>[4x]MSDKTKTNEGFSRRSFIGSAAVVTAGVAGLGAIDAASATQKTNRASTVKGGFDYD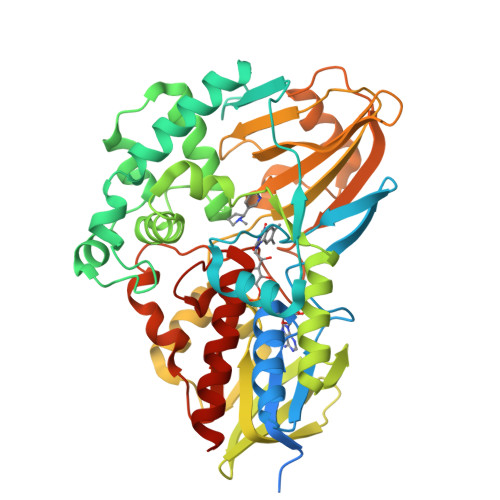VVVVGGGFAGATAARECGLQGYRTLLLEARSRLGGRTFTSRFAGQEIEFGGAWVHWLQPHVWAEMQRYGLGVVEDPLTNLDKTLIMYNDGSVESISPDEFGKNIRIAFEKLCHDAWEVFPRPHEPMFTERARELDKSSVLDRIKTLGLSRLQQAQINSYMALYAGETTDKFGLPGVLKLFACGGWNYDAFMDTETHYRIQGGTIGLINAMLTDSGAEVRMSVPVTAVEQVNGGVKIKTDDDEIITAGVVVMTVPLNTYKHIGFTPALSKGKQRFIKEGQLSKGAKLYVHVKQNLGRVFAFADEQQPLNWVQTHDYSDELGTILSITIARKETIDVNDRDAVTREVQKMFPGVEVLGTAAYDWTADPFSLGAWAAYGVGQLSRLKDLQAAEGRILFAGAETSNGWHAVIDGAVESGLRAGREVKQLLSLEHHHHHH>[4x]EDNSLSQKKKVTVEDLFSEDFKIHDPEAKWISDTEFIYREQKGTVRLWNVETNTSTVLIEGKKIESLRAIRYEISPDREYALFSYNVEPIYQHSYTGYYVLSKIPHGDPQSLDPPEVSNAKLQYAGWGPKGQQLIFIFENNIYYCAHVGKQAIRVVSTGKEGVIYNGLSDWLYEEEILKTHIAHWWSPDGTRLAYAAINDSRVPIMELPTYTGSIYPTVKPYHYPKAGSENPSISLHVIGLNGPTHDLEMMPPDDPRMREYYITMVKWATSTKVAVTWLNRAQNVSILTLCDATTGVCTKKHEDESEAWLHRQNEEPVFSKDGRKFFFIRAIPQGGRGKFYHITVSSSQPNSSNDNIQSITSGDWDVTKILAYDEKGNKIYFLSTEDLPRRRQLYSANTVGNFNRQCLSCDLVENCTYFSASFSHSMDFFLLKCEGPGVPMVTVHNTTDKKKMFDLETNEHVKKAINDRQMPKVEYRDIEIDDYNLPMQILKPATFTDTTHYPLLLVVDGTPGSQSVAEKFEVSWETVMVSSHGAVVVKCDGRGSGFQGTKLLHEVRRRLGLLEEKDQMEAVRTMLKEQYIDRTRVAVFGKDYGGYLSTYILPAKGENQGQTFTCGSALSPITDFKLYASAFSERYLGLHGLDNRAYEMTKVAHRVSALEEQQFLIIHPTADEKIHFQHTAELITQLIRGKANYSLQIYPDESHYFTSSSLKQHLYRSIINFFVECFRI

Modulation of voltage-gated potassium (Kv) channels by auxiliary subunits is central to the physiological function of channels in the brain and heart. Native Kv4 tetrameric channels form macromolecular ternary complexes with two auxiliary β-subunits—intracellular Kv channel-interacting proteins (KChIPs) and transmembrane dipeptidyl peptidase-related proteins (DPPs)—to evoke rapidly activating and inactivating A-type currents, which prevent the backpropagation of action potentials. Here we report cryo-electron microscopy structures of the Kv4.2–DPP6S–KChIP1 dodecamer complex, the Kv4.2–KChIP1 and Kv4.2–DPP6S octamer complexes, and Kv4.2 alone. Thus, our data suggest that two distinct modes of modulation contribute in an additive manner to evoke A-type currents from the native Kv4 macromolecular complex.

The 3D classes that contained four DPP6S molecules were selected for further 3D refinement with C2 symmetry imposed, because two DPP6S dimers were integrated with C2 symmetry in the complexes. Owing to the flexible position of the large extracellular domains of DPP6S floating above Kv4.2, the overall resolutions are 4.2 Å and 4.5 Å for the Kv4.2–DPP6S and Kv4.2–DPP6S–KChIP1 complexes, respectively. The dimeric crystal structure of the DPP6S extracellular domain43 was used as a guide to construct the atomic models of the Kv4.2–DPP6S and Kv4.2–DPP6S–KChIP1 structures. In the extracellular region, two DPP6S dimers float above the channel core.> MAFISSGYNPAKPMENRITDIGPRKFTEFFPPVIAKNAGNWDYHEILEPGILVHVAKNGDKVFTVRCGAARLMSTSHIREACEIAKKFCNGHLRFTTRNNIEFMVDNEETLKALVADLKTRKFAAGSFKFPIGGTGASISNIVHTQGWVYCHTPATDASGPVKAVMDELFEEFTSMRLPAIVRVSLACCINMCGAVHCSDIGLVGIHRKPPMIDHE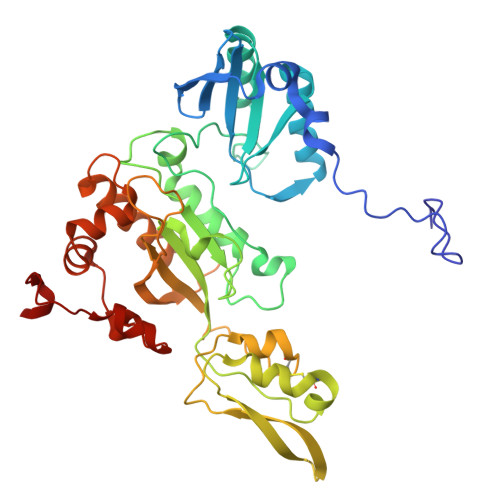NLAELCEIPLAVAACPTAAVKPITAEVNGQKVKSVAINNDRCMYCGNCYTMCPALPLSDGTGDGIAIMVGGKISNRIKVPSFSKVVVAFVPNEPPRWPTMAKIVKKIVEVYAEDARKYERIGDWIHRIGWETFYEKTGLEFSHHCIDDFRDPAYYTWRQSTQFKFVSFDS>[4x]MHHHHHHKGFAMLSIGKVGWIEKEKPAPGPFDAIVRPLAVAPCTSDITTVFEGAIGERHNM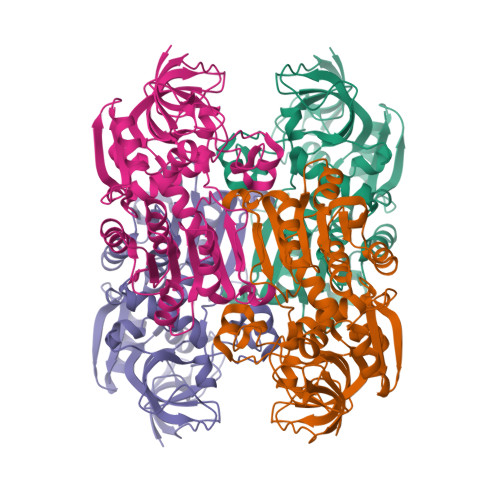ILGHEAVGEVVEVGSEVKDFKPGDRVVVPGATPDWRTSEVQRGYHQHSGGMLAGWKFSNVKDGVFGEFFHVNDADMNLAHLPKEIPLEAAVMIPDMMTTGFHGAELADIELGATVAVLGIGPVGLMAVAGAKLRGAGRIIAVGSRPVCVDAAKYYGATDIVNYKDGPIESQIMNLTEGKGVDAAIIAGGNADIMATAVKIVKPGGTIANVNYFGEGEVLPVPRLEWGCGMAHKTIKGGLCPGGRLRMERLIDLVFYKRVDPSKLVTHVFRGFDNIEKAFMLMKDKPKDLIKPVVILA> GPSRGAQNSISWEVQRFDGWYNNLMEHRWGSKGSRLQRLVPAS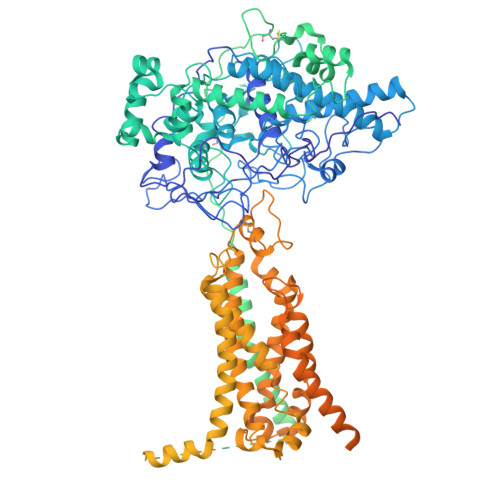YADGVYQPLKEPYLPNPRHLSNRVMRGSAGQPSLRNRTVLGVFFGYHVLSDLVSVETPGCPAEFLNIYIPHGDPVFDPDKRGNVVLPFQRSRWDRNTGQSPSNPRDQSNQVTGWLDGSAIYGSSHSWSDTLRSFSGGQLASGPDPAFPSDSQSSLLMWMAPDPSTGQGGPRGVYAFGAQRGNREPFLQALGLLWFRYHNLCARKLAQEHPHWGDEELFQHARKRVIATYQNIAMYEWLPSFLKQTPPEYPGYRPFLDPSISPEFVVASEQFLSTMVPSGVYMRNASCHFQGIPSHNSSVSGALRVCNSYWSREHPKLQRAEDVDALLLGMASQIAEREDHVVVEDMQDFWPGPLKFSRTDYLASCLQRGRDLGLPSYTKAREALGLSPISHWQDINPALSRSNGTVLEATAALYNQDLSRLELLPGGLLESHGDPGPLFSTIVLDQFVRLRDGDRYWFENTRNGLFSKEEIAEIRNTSLRDILVAVTNVDPSALQPNVFFWLAGDPCPQPSQLSAKGLPACAPLFIRDYFEGSGFGFGLTIGTLCCFPLVSLLSAWIVARLRKRNFKRLQRQDRQSIMSEKLVGGVEALEWQGRNEPCRPVLVHLQPGQIRVVDGRLTVLRTIQLRPPQQVNLILSSNRGRRTLLLKIPKEYDLVLLFNMEEERQALVENVRGALKENGLSFQEWELREQELMRAAVTRQQRGHLLETFFRHLFSQVLDINQADAGTLPLDSSTKVREALTCELSRAEFADSLGLKPQDMFVESMFSLADKDGNGYLSFREFLDILVVFMKGSPEEKSRLMFRMYDFDGNGLISKDEFIRMLRSFIEISNNCLSKAQLAEVVESMFRESGFQDKEELTWEDFHFMLRDHDSDLRFTQLCVKGVEVPEVIKNLCRRASYISQEKICPSPRMSAHCARNNMKTASSPQRLQCPMDTDPPQEIRRRFGKKVTSFQPLLFTEAHREKFQRSRRHQTVQQFKRFIENYRRHIGCVAVFYTITGALFLERAYYYAFAAHHSGITDTTRVGIILSRGTAASISFMFSYILLTMCRNLITFLRETFLNRYIPFDAAVDFHRLIASTAIILTVLHSAGHVVNVYLFSISPLSVLSCLFPGLFHDDGSEFPQKYYWWFFQTVPGLTGVLLLLALAIMYVFASHHFRRRSFRGFWLTHHLYIFLYILLIIHGSFALIQMPRFHIFFLVPAIIYVGDKLVSLSRKKVEISVVKAELLPSGVTHLRFQRPQGFEYKSGQWVRIACLALGTTEYHPFTLTSAPHEDTLSLHIRAAGPWTTRLREIYSPPTGDTCARYPKLYLDGPFGEGHQEWHKFEVSVLVGGGIGVTPFASILKDLVFKSSVSCQVFCKKIYFIWVTRTQRQFEWLADIIREVEENDRQDLVSVHIYITQLAEKFDLRTTMLYICERHFQKVLNRSLFTGLRSITHFGRPPFEPFFNSLQEVHPQVRKIGVFSCGPPGMTKNVEKACQLINRQDRTHFSHHYENF2-(4-chlorophenoxy)-N-{[(4R)-4-methyl-2,5-dioxoimidazolidin-4-yl]methyl}acetamide 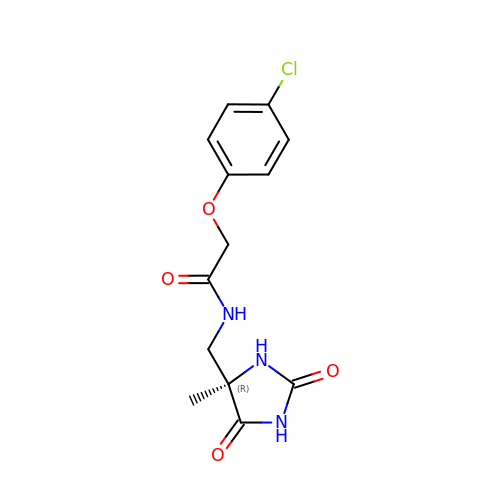| C13 H14 Cl N3 O4 | LNIRXDCIYOBRPL-CYBMUJFWSA-N> GSGIVPQLQNIVSTVNLGCKLDLKTIALRAR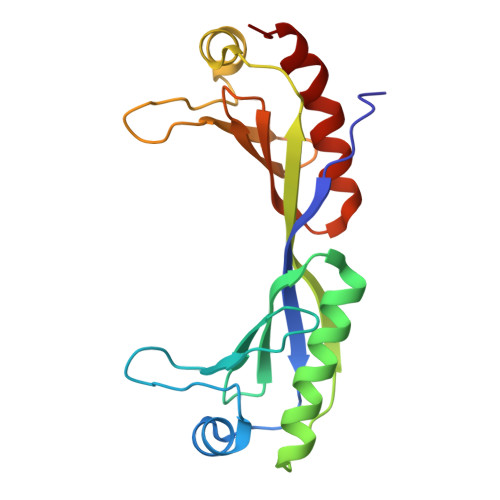NAEYNPKRFAAVIMRIREPRTTALIFSSGKMVCTGAKSEEQSRLAARKYARVVQKLGFPAKFLDFKIQNMVGSCDVKFPIRLEGLVLTHQQFSSYEPELFPGLIYRMIKPRIVLLIFVSGKVVLTGAKVRAEIYEAFENIYPILKGFRK The curli biogenesis system in Enterobacteriaceae such as Salmonella species and Escherichia coli (E.coli), also known as the nucleation-precipitation or type VIII secretion system, is responsible for secreting curli subunits into the extracellular milieu to form cell associated nonbranching and highly aggregative amyloid fibrils. Lipoprotein CsgG forms a nonameric secretion channel in the outer membrane and transports CsgA and CsgB from periplasm into extracellular environment. Two soluble accessory factors, CsgE and CsgF, have been thought to bind to CsgG and play a crucial role in substrate (CsgA and CsgB) secretion and curli amyloid fiber formation. To address these questions, we determined the structures of complexes in curli biogenesis system by electron cryo-microscopy (cryoEM), including CsgF and CsgG (CsgFG) complexes both in the free for and bound to the N terminus (residues 1–22) of CsgA (CsgAN22).

To investigate how CsgAN22 binds to the CsgFG complex, we determined the cryoEM structure of the CsgFG-CsgAN22 complex with an imposed C9 symmetry at 3.34 Å resolution. The overall architecture of CsgFG-CsgAN22 complex was nearly identical to that of CsgFG complex. The differences of CsgFG-CsgAN22 complex from CsgFG complex include two additional densities on each CsgG subunit outside the CsgG periplasmic chamber. One being a part of CsgAN22 (residues 2–7, sequence VVPQYG) and the other being a CsgG loop (residues 104–110) missing in the CsgFG complex in the absence of CsgAN22. This loop was found to be flexible in CsgFG complex and stabilized after binding to CsgAN22. Six CsgAN22 residues (V2V3P4Q5Y6G7) were trapped in a crevice on CsgG surface mainly by hydrophobic interactions and hydrogen-bonds. Using multiple sequence alignment (MSA), we found that the Val3 residue of CsgA was conserved and interacted with a small hydrophobic pocket surrounded by residues I121, L172, L236, and W237 of CsgG. Gln5 residue is highly conserved as shown by MSA and forms hydrogen-bonds with the main-chain residues Asp238 and Gly32 residues and side chain of Thr31 of CsgG. Tyr6 interacts with the CsgG subunit to stabilize the adjacent CsgG loop region (residues 107–110). Altogether, we found that CsgG recognizes CsgA mainly by binding to the conserved residues Val3, Gln5, and Tyr6.

>MQRLFLLVAVMLLSGCLTAPPKEAARPTLMPRAQSYKDLTHLPAPTGKIFVSVYNIQDETGQFKPYPASNFSTAVPQSATAMLVTALKDSRWFIPLERQGLQNLLNERKIIRAAQENGTVAINNRIPLQSLTAANIMVEGSIIGYESNVKSGGVGARYFGIGADTQYQLDQIAVNLRVVNVSTGEILSSVNTSKTILSYEVQAGVFRFIDYQRLLEGEVGYTSNEPVMLCLMSAIETGVIFLINDGIDRGLWDLQNKAERQNDILVKYRHMSVPPES[9x];>[9x]MRVKHAVVLLMLISPLSWAGTMTFQFRNPNFGGNPNNGAFLLNSAQAQNSYKDPSYNDDFGIETPSALDNFTQAIQSQILGGLLSNINTGKPGRMVTNDYIVDIANRDGQLQLNVTDRKTGQTSTIQVSGLQNNSTDF;>GVVPQYGGGGNHGGGGNNSGPN[9x]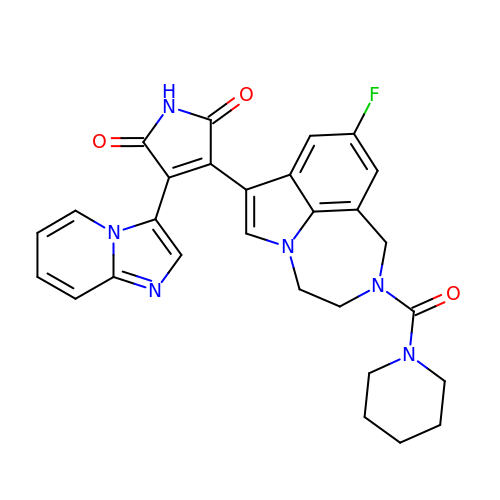LY-2090314 | C28 H25 F N6 O3 | HRJWTAWVFDCTGO-UHFFFAOYSA-N>[2x]AEFKHVFVCVQDRPPGHPQGSCAQRGSREVFQAF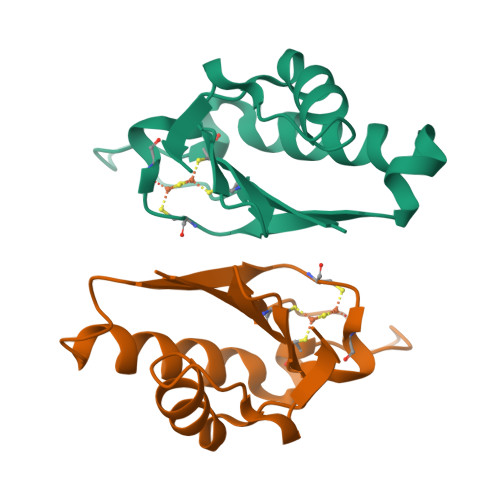MEKIQTDPQLFMTTVITPTGCMNASMMGPVVVVYPDGVWYGQVKPEDVDEIVEKHLKGGEPVERLVISKGKPPGMF> MMDLNNAYDHCKNIIEKHSKTFSKAFAMLPKHQKRAVWAIYAFCRRADDIVDEGENPKEELEAFAVEFDLFMEGRLETEDPCWIALQDAFERFPLDPAPFYEMIVGQRMDLYPKTIDTKDDLLHYCYHVASTVGLMLLPVLAPGKVSRVKTGAIELGYAMQITNILRDIGEDLD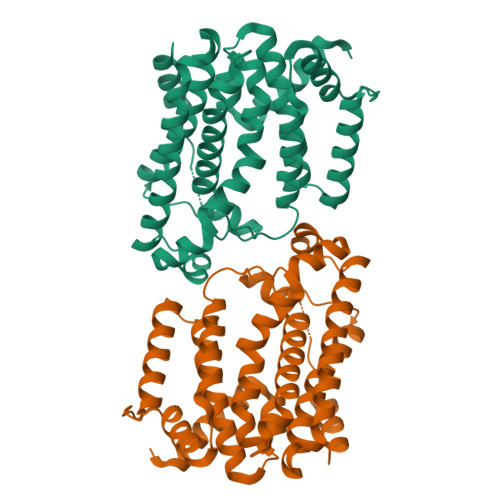NHRIYIPKQMMIEYGYTRTDLHNKKVNEAFIQLWEDLAQDAEHYYRNALATLPEYPVYSRTPVGGAAKMYRAIIQTVRNNDYQVFGKRNYVSDQMKKQIIAEMQ> MRGSHHHHHHGSLVPRGSNTYGWDIVYGCSNRVVNKHLKNYIDENKIEFLYSDINKKQEIKMIFDNWEIINGGTSNFLRIKIFIKEGYFKFRNTTVDLSGVIPILEIKLDFFNDASNPHIKELKFS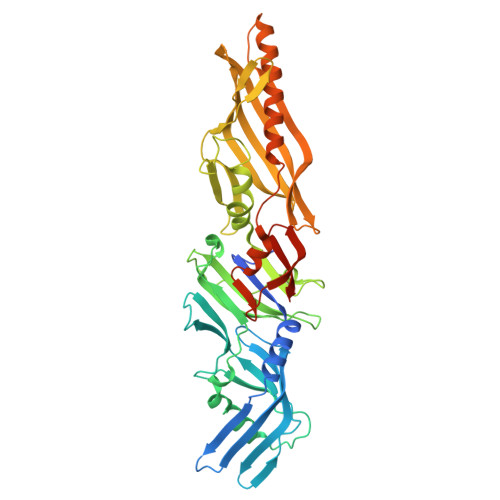FGNKTNDDIKVIVSDLSGKLYEEDEFYFNKLLISAFINNEKQVSYIFASLNVTSNIVWMNPKQFKFVYYSPTDNNDGYLCILSVVTNRDISKLSTNVDSSILSENSEVGLLISEKLFMENLLLPKLSSNMGSNITSNNFNVINTSDTTGIIKNKNTLNWYGIKVAALYYYPEINDFSMELFEGNKLKTRLSGIVKLTGYERIYSKLNMECITKFIYDNKNKKVSFEIYSTPIMECRPIFGLLDGIPAAVAKSVGNWSLKSFRDSLAFELANNFTDIINDIVNWNNLKISEVTNIILNVGFCIQGNMNPGSAWSHPQFEK> GSGSDEKICAIYPHLKDSYWLSVNYGMVSEAEKQGVNLRVLEAGGYPNKSRQEQQLALCTQWGANAIILGTVDPHAYEHNLKSWVGNTPVFATVNQLDL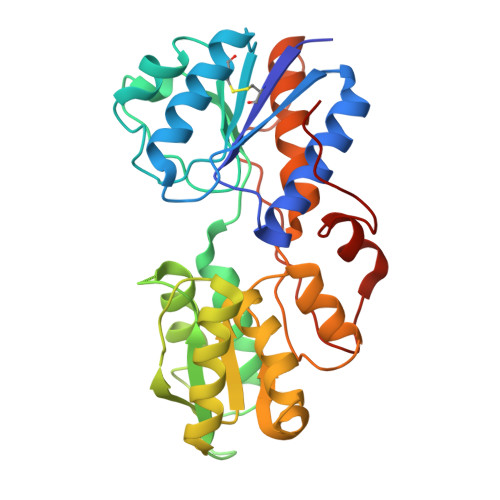DEEQSTLLKGEVGVDWYWMGYEAGKYLAERHPKGSGKTNIALLLGPRTRGGTKPVTTGFYEAIKNSDIHIVDSFWADNDKELQRNLVQRVIDMGNIDYIVGSAVAIEAAISELRSADKTHDIGLVSVYLSHGVYRGLLRNKVLFAPTDKMVQQGRLSVMQAAHYLRHQPYEKQASPIIKPLTPKTLHDDTIEESLSPSEYRPTFS(1~{R})-1-[10-[3-(dimethylamino)propyl]phenothiazin-2-yl]ethanol 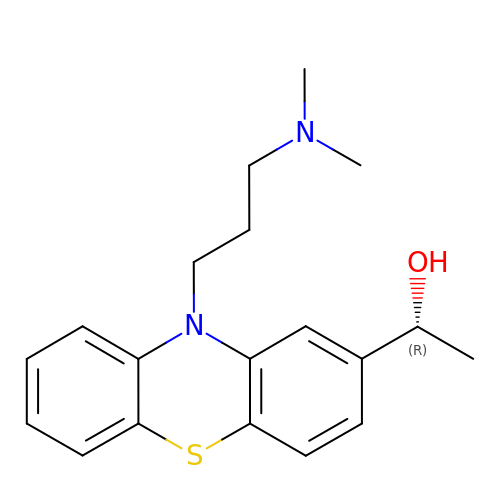| C19 H24 N2 O S | ZIJWCRNUEBJMSQ-CQSZACIVSA-N>[2x]GC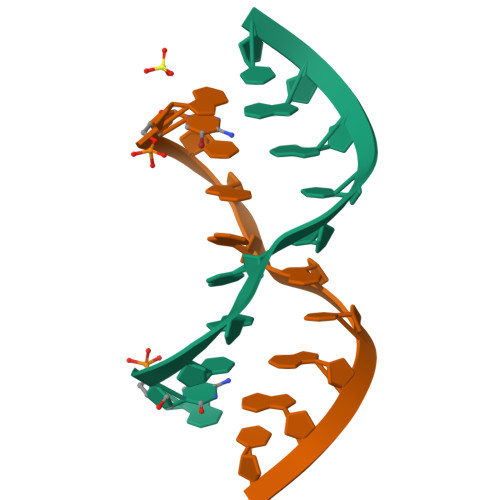CGGAUGGC> AGAGCGUUGCGUCCGAAAGUCGCC;> GCGACACGGCUCUUUAAAAACAAAAG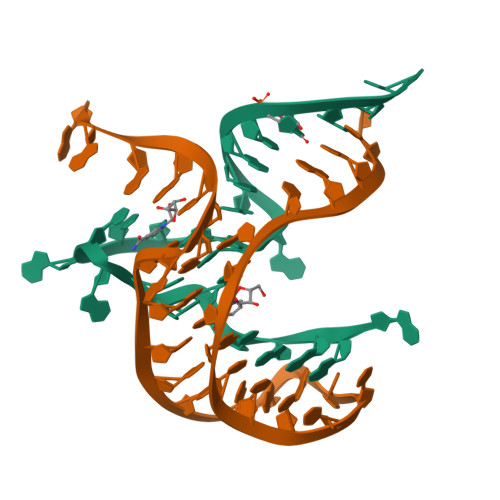GAGAA> GPMDTKFKDDLFRKYVQFHESKVDTTTSRQRPGSDECLRVAASTLLSLHKVDPFYRFRLIQFYEVVESSLRSLSSSSLRALHGAFSMLETVGINLFLYPWKKEFRSIKTYTGPFVYYVKSTLLEEDIRAILSCMGYTPELGTAYKLRELVETLQVKMVSFELFLAKVECEQMLEIHSQVKDKGYSELDIVSERKSSAEDVRGCSDALRRRAEGRE

The linear ubiquitin chain assembly complex (LUBAC) regulates immune signaling, and its function is regulated by the deubiquitinases OTULIN and CYLD, which associate with the catalytic subunit HOIP. We here show that CYLD interacts with HOIP via spermatogenesis-associated protein 2 (SPATA2). SPATA2 interacts with CYLD through its non-canonical PUB domain, which binds the catalytic CYLD USP domain in a CYLD B-box-dependent manner. SPATA2 also harbors a conserved PUB-interacting motif that selectively docks into the HOIP PUB domain.

A crystal structure of the SPATA2 PUB domain (aa 7–219) at 1.45 Å resolution revealed a fold most similar to that of the extended PUB domain in HOIP (root-mean-square deviation [RMSD] 2.4 Å) (Elliott et al., 2014) and the smaller PUB domain of PNGase (RMSD 3.2 Å) (Zhao et al., 2007). Species conservation of SPATA2 mapped onto the surface of the PUB domain reveals that while the PIM pocket is highly conserved, this interaction site is also very different from canonical PUB domains. The previously mapped PUB-PIM interactions include a conserved Asp-Leu/Met-Tyr (see below), in which Leu and Tyr occupy a deep, hydrophobic gorge on the PUB surface, the PIM pocket. In SPATA2, this pocket is significantly different from both HOIP as well as PNGase structures, and modeling of interactions with PIM peptides derived from OTULIN or p97 would generate steric clashes. Consistently, the SPATA2 PUB domain does not bind PIM peptides (see below), suggesting an interaction motif in CYLD may need to display distinct properties. Nonetheless, the high conservation in this area did suggest that this surface may mediate CYLD interactions, and single amino acid mutations in or near the SPATA2 PIM pocket interfered with CYLD binding. In particular, mutations in the “lower wall” of the SPATA2 PIM pocket (Y114A, T115N, and T115A) decreased CYLD interactions, while mutation of residues in the “upper wall” of the pocket (N98A and T94K) did not have strong effects on CYLD binding. The strongest effect on CYLD binding was observed when we mutated Tyr114, which points away from the PIM pocket, supporting that CYLD binds the SPATA2 PUB domain in a PIM-independent manner. Indeed, the CYLD USP domain (aa 583–956) and SPATA2 PUB domain (aa 1–241) formed an SEC-stable complex, confirming a direct interaction.> NLIPTVIEQTNRGERAYDIYS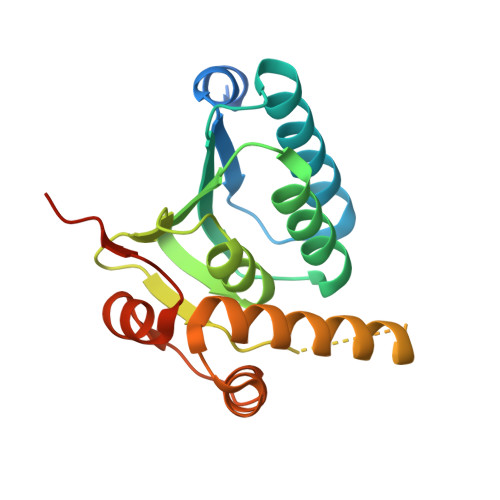RLLKDRIIMLGSAIDDNVANSIVSQLLFLAAEDPEKEISLYINSPGGSITAGMAIYDTMQFIKPKVSTICIGMAASMGAFLLAAGEKGKRYALPNSEVMIHQPLGGAQGQATEIEIAAKRILLLRDKLNKVLAERTGQPLEVIERDTDRDNFKSAEEALEYGLIDKILTHLEHHHHHH(10R,13S)-16-amino-13-hydroxy-7,13-dioxo-8,12,14-trioxa-13lambda~5~-phosphahexadecan-10-yl tridecanoate | C25 H50 N O8 P | 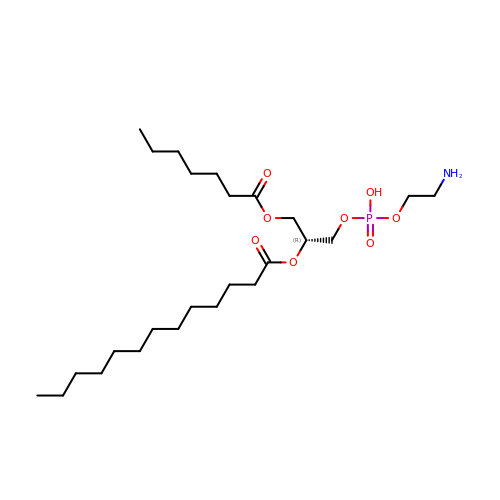DZBORIDLQAEVCV-HSZRJFAPSA-N The Ca2+-binding photoprotein aequorin is a complex of apoAequorin (apoprotein) and (S)-2-peroxycoelenterazine. apoAequorin, which consists of 189 amino acid residues, can be regenerated to aequorin by incubation with coelenterazine and O2, both in vivo and in vitro. The chiral deaza-analogs of (S)-daCTZ and (S)-HM-daCTZ selectively inhibited the regeneration step to aequorin by binding the catalytic site of coelenterazine in the apoAequorin molecule. The crystal structures of the apoAequorin complexes with (S)-daCTZ and (S)-HM-daCTZ were determined, suggesting that the hydroxy moiety at the C6-hydroxyphenyl group and the carbonyl moiety of the imidazopyrazinone ring in coelenterazine are essential to bind the apoAequorin molecule through hydrogen bonding.

As the deaza-analogs of (S)-daCTZ and (S)-HM-daCTZ were regarded as coelenterazine and (S)-2-peroxycoelenterazine, respectively, (S)-daCTZ could be used as a probe to determine the recognition residues of apoAequorin and (S)-HM-daCTZ could be applied to confirm the binding environment of (S)-2-peroxycoelenterazine in apoAequorin, as previously reported. Because the chirality at the C2-peroxy moiety of 2-peroxycoelenterazine in aequorin is the S form, (S)-HM-daCTZ showed strong inhibition on the regeneration to aequorin, but not (R)-HM-daCTZ. The strong inhibition of (S)-daCTZ and (S)-HM-daCTZ on aequorin regeneration indicate that the deaza-analogs can generate a stable complex with apoAequorin. Native aequorin consists of apoAequorin and (S)-2-peroxycoelenterazine, and the (S)-2-peroxy group is stabilized by the hydrogen-bonding interaction with the hydroxy group of Tyr184. Similarly, in the apoAequorin/(S)-HM-daCTZ complex, the hydroxymethyl group at the C2 position of (S)-HM-daCTZ and the C3-carbonyl moiety were stabilized with Tyr184 and His169, respectively. Also, the hydroxy moiety at the C6-hydroxyphenyl group was stabilized with His16, Tyr82, and Trp86, identical to that of native aequorin. The absorption spectrum of the apoAequorin/(S)-HM-daCTZ complex was distinct from that of native aequorin, which consisted of (S)-2-peroxycoelenterazine and apoAequorin. Furthermore, the addition of Ca2+ to the apoAequorin/(S)-HM-daCTZ complex did not affect the absorption spectrum significantly. As a result, the apoAequorin/(S)-HM-daCTZ complex was converted to aequorin, exhibiting the Ca2+-triggered flash luminescence.

>ANSHHHHHHGKLTSDFDNPRWIGRHKHMFNFLDVNHNGKISLDEMVYKASDIVINNLGATPEQAKRHKDAVEAFFGGAGMKYGVETDWPAYIEGWKKLATDELEKYAKNEPTLIRIWGDALFDIVDKDQNGAITLDEWKAYTKAAGIIQSSEDCEETFRVCDIDESGQLDVDEMTRQHLGFWYTMDPACEKLYGGAVP[16x]>[2x]PIISAEDKHLTVLNLFTTDTPEKQGKLIEEMTKIVDAATYEGWMSSTVHSGVDSHGTLNFIQWRSGEDLEKRYAGEEFKHRTLP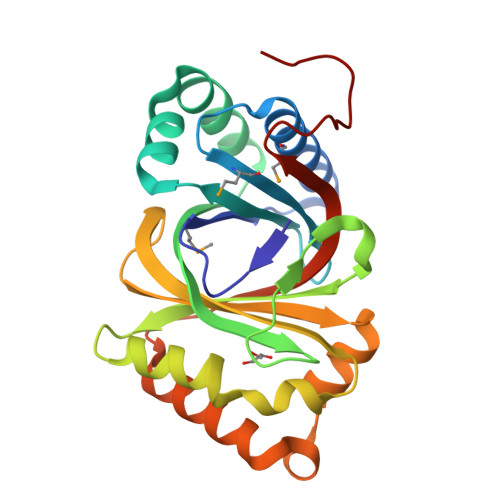VFGEITTSIRLMQNEVAHTLTSDALGGKIEIGPGRDDYTVFTVFPVTPQGQDEALDALGPGQAFLAQVPGFRAHVVLKGLRARGLEGAFVISYSQWDSKQAWEAYRDQAPQDQDEARKAAVGRVRAVVAGEPYSNTYQVVHTRSAGEKLAAALEHHH ADENOSINE-5'-DIPHOSPHATE-2-DEOXY-2-FLUORO HEPTOSE | C17 H26 F N5 O15 P2 | 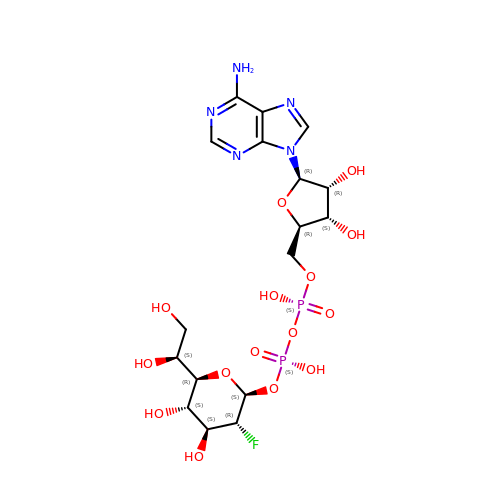SUPCMUQXGKOKIM-FJBXLJLUSA-N>[2x]LAFGAIQLDGDGNILQYNAAEGD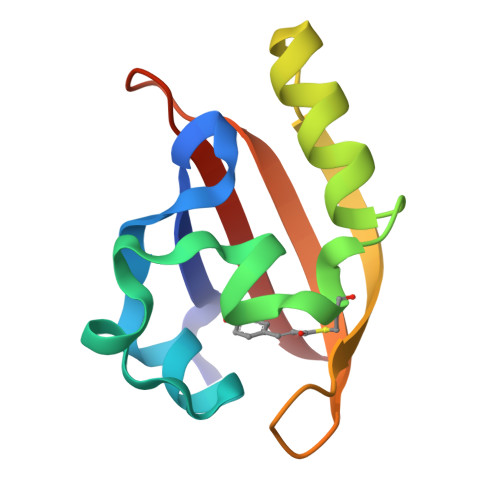ITGRDPKQVIGKNFFKDVAPCTDSPEFYGKFKEGVASGNLNTMFEYTFDYQMTPTKVKVHMKKALSGDSYWVFVKRV> A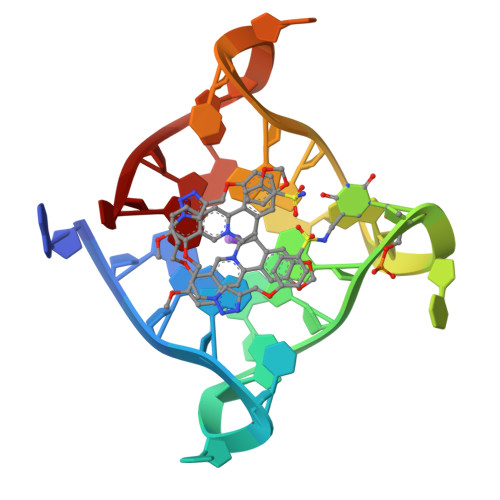GGGTTAGGGTTAGGGTTAGGGT>QFTDIDKLAVSTIRILAVDTVSKANSGHPGAPLGMAPAAHVLWSQMRMNPTNPDWINRDRFVLSNGHAVALLYSMLHLTGYDLSIEDLKQFRQLGSRTPGHPEFELPGVEVTTGPLGQGISNAVGMAMAQANLAATYNKPGFTLSDNYTYVFLGDGCLQEGISSEASSLAGHLKLGNLIAIYDDNKITIDGATSISFDEDVAKRYEAYGWEV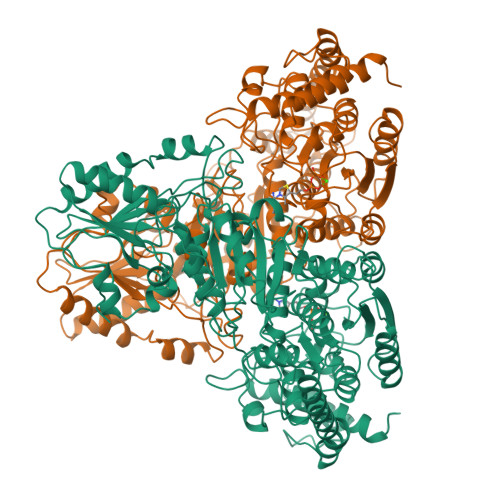LYVENGNEDLAGIAKAIAQAKLSKDKPTLIKMTTTIGYGSLHAGSHSVHGAPLKADDVKQLKSKFGFNPDKSFVVPQEVYDHYQKTILKPGVEANNKWNKLFSEYQKKFPELGAELARRLSGQLPANWESKLPTYTAKDSAVATRKLSETVLEDVYNQLPELIGGSADLTPSNLTRWKEALDFQPPSSGSGNYSGRYIRYGIREHAMGAIMNGISAFGANYKPYGGTFLNFVSYAAGAVRLSALSGHPVIWVATHDSIGVGEDGPTHQPIETLAHFRSLPNIQVWRPADGNEVSAAYKNSLESKHTPSIIALSRQNLPQLEGSSIESASKGGYVLQDVANPDIILVATGSEVSLSVEAAKTLAAKNIKARVVSLPDFFTFDKQPLEYRLSVLPDNVPIMSVEVLATTCWGKYAHQSFGIDRFGASGKAPEVFKFFGFTPEGVAERAQKTIAFYKGDKLISPLKKAF[2x]> HHHHHHASENLYFQGAMVMASEKHFKYVILGGGVAAGYAAREFAKQGVKPGELAIISKEAVAPYE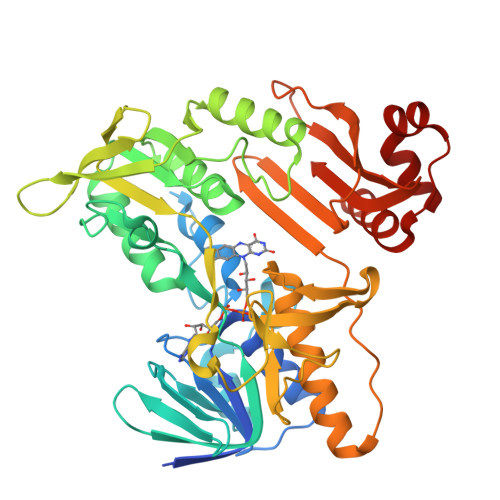RPALSKGYLFPQNAARLPGFHVCVGSGGERLLPEWYSEKGIELILSTEIVKADLASKTLTSAVGATFTYEILIIATGSSVIKLSDFGTQGADSNNILYLREVDDADKLVAAIQAKKGGKAVIVGGGYIGLELSAALKINDFDVTMVFPEPWCMPRLFTADIAAFYESYYTNKGVKIVKGTVAVGFDADANGDVTAVNLKNGSVLEADIVVVGVGGRPLTTLFKGQVAEEKGGIKTDAFFETSVPGVYAVGDVATFPMKMYNELRRVEHVDHARKSAEQAVKAIKGKESGESVVEYDYLPYFYSRSFDLGWQFYGDNVGDTILFGDSDPTSAKPKFGSYWIKDGKVLGAFLEGGSPDENKAIAKVAKTQPPVANIEELKKEGLQFASKI5-(5-FLUORO-2-METHYLPHENYL)-6,7,8,9-TETRAHYDRO-3H-PYRAZOLO[3,4-C]ISOQUINOLIN-1-AMINE | C17 H17 F N4 | 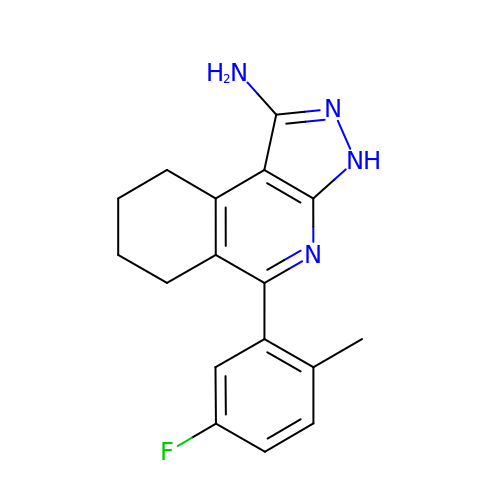YPULTKAHHAYKOE-UHFFFAOYSA-N>MKLYTKTGDKGQTGLVGGRTDKDSLRVESYGTIDELNSFIGLALAELSGQPGFEDLTAELLTIQHELFDCGGDLAIVTERKDYKLTEESVSFLETRIDAYTAEAPELKKFILPGGSKCASLLHIARTITRRAERRVVALMKSEEIHETVLRYLNRLSDYF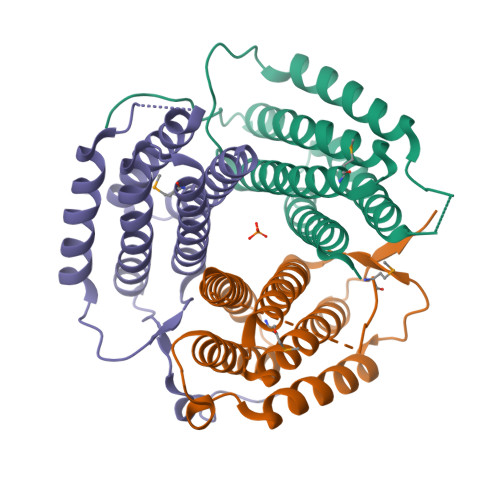FAGARVVNARSGIGDVEYERSAIVFRDRNSSES[3x]>[2x]PSQMEHAMETMMFTFHKFAGDKGYLTKEDLRVLMEKEFPGFLENQKDPLAVDKI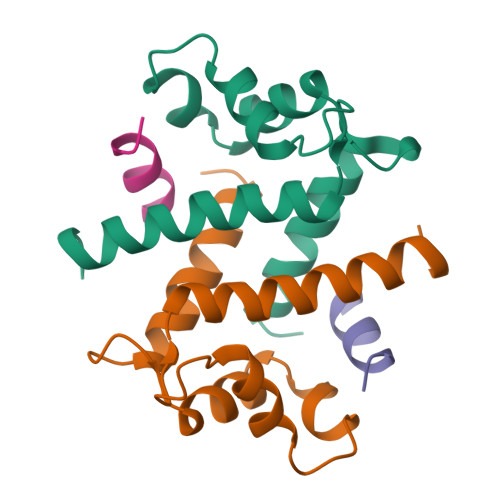MKDLDQCRDGKVGFQSFFSLIAGLTIACNDYFVVHMKQKGKK;>[2x]XSTVHEILSKLSLE(3S)-3-{4-[3-(4-fluorophenyl)-1-methyl-1H-pyrazol-4-yl]pyridin-2-yl}morpholine 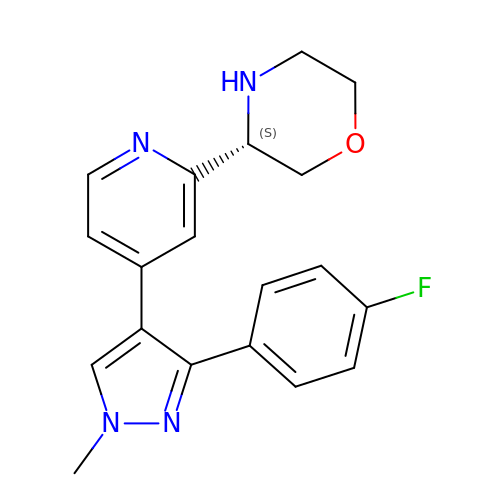| C19 H19 F N4 O | ZVSNVLKUNCNJEG-GOSISDBHSA-N> MDYKDDDDKPNPPSFKSHKQNLFNSNNNQHANSVDSFDLHLDDSFDAALDSLQINNNPEPLSKHNTVGDRESFEMRTVDDLDNFSNHSSDSHRKSSNTDTHPLMYDNRLSQDDNFKFTNIASSPPSSSNNIFSKALSYLKVSNTKNWSKFGSPIELSDQHIEREIHPDTTPVYDRNRYVSNELSNAKYNAVTFVPTLLYEQFKFFYNLYFLVVALSQAVPALRIGYLSSYIVPLAFVLTVTMAKEAIDDIQRRRRDRESNNELYHVITRNRSIPSKDLKVGDLIKVHKGDRIPADLVLLQSSEPSGESFIKTDQLDGETDWKLRVACPLTQNLSENDLINRISITASAPEKSIHKFLGKVTYKDSTSNPLSVDNTLWANTVLASSGFCIACVVYTGRDTRQAMNTTTAKVKTGLLELEINSISKILCACVFALSILLVAFAGFHNDDWYIDILRYLILFSTIIPVSLRVNLDLAKSVYAHQIEHDKTIPETIVRTS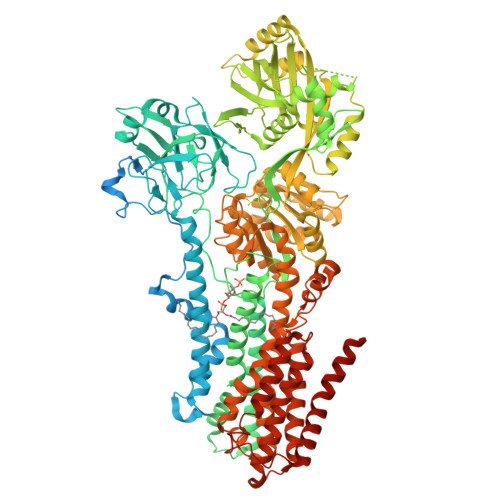TIPEDLGRIEYLLSDKTGTLTQNDMQLKKIHLGTVSYTSETLDIVSDYVQSLVSSKNDSLNNSKVALSTTRKDMSFRVRDMILTLAICHNVTPTFEDDELTYQAASPDEIAIVKFTESVGLSLFKRDRHSISLLHEHSGKTLNYEILQVFPFNSDSKRMGIIVRDEQLDEYWFMQKGADTVMSKIVESNDWLEEETGNMAREGLRTLVIGRKKLNKKIYEQFQKEYNDASLSMLNRDQQMSQVITKYLEHDLELLGLTGVEDKLQKDVKSSIELLRNAGIKIWMLTGDKVETARCVSISAKLISRGQYVHTITKVTRPEGAFNQLEYLKINRNACLLIDGESLGMFLKHYEQEFFDVVVHLPTVIACRCTPQQKADVALVIRKMTGKRVCCIGDGGNDVSMIQCADVGVGIVGKEGKQASLAADFSITQFCHLTELLLWHGRNSYKRSAKLAQFVMHRGLIIAICQAVYSICSLFEPIALYQGWLMVGYATCYTMAPVFSLTLDHDIEESLTKIYPELYKELTEGKSLSYKTFFVWVLLSLFQGSVIQLFSQAFTSLLDTDFTRMVAISFTALVVNELIMVALEIYTWNKTMLVTEIATLLFYIVSVPFLGDYFDLGYMTTVNYYAGLLVILLISIFPVWTAKAIYRRLHPPSYAKVQEFATP> AKCVSYGVSQIKAPALHSQGYTGSNVKVAVIDSGIDSSHPDLNVAGGASFVPSETNPFQDNNSHGTHVAGTVLAVAPSASLYAVKVLGADGSGQYSWIINGIEWAIANNMDVINMSLGGPSGSAALKAAVDKAVASGVVVVAAAGNSGTSGSSSTVSYPAKYPSVIAVGAVDSSNQRAPFSSVGPELDVMAPGVSICSTLPGNKYGALSGTCPASAHVAGAAALILSKHPNWTNTQVRSSLENTATKLGDSFYYGKGLINVEAAAQHHHHHH

Omniligase-1 is a broadly applicable enzyme for peptide bond formation between an activated acyl donor peptide and a non-protected acyl acceptor peptide. The enzyme is derived from an earlier subtilisin variant called peptiligase by several rounds of protein engineering aimed at increasing synthetic yields and substrate range. Mutation A225N in the S1′ pocket and F189W of the S2′ pocket increased the synthesis to hydrolysis (S/H) ratio and overall coupling efficiency, whereas the I107V mutation was added to S4 pocket to increase the reaction rate. The final omniligase variants appeared to have a very broad substrate range, coupling more than 250 peptides in a 400-member library of acyl acceptors, as indicated by a high-throughput FRET assay.

Inspection of the crystal contacts of Pre-1, Pre-2 and Pre-3 revealed that at position F189 (S2′ pocket) the enzymes in crystal form A as well as in crystal form B have close contact (3.7 Å) with Asn109 of a symmetry-related molecule. A Trp instead of a Phe at position 189 would be too close to this Asn (2.0 Å W189-CD1 to ND1 or OD1 of N109) which cannot adopt a different conformation because of steric hindrance. Thus, Oml-1 and other omniligase variants containing mutation F189W, which is crucial for the broad substrate scope, cannot be crystallized in crystal form A or B.~{N}-[[4-[[(2~{S})-4-cyclohexyl-1-[[(3~{S})-1-methylsulfonylpiperidin-3-yl]amino]-1-oxidanylidene-butan-2-yl]carbamoyl]phenyl]methyl]imidazo[1,2-a]pyridine-3-carboxamide 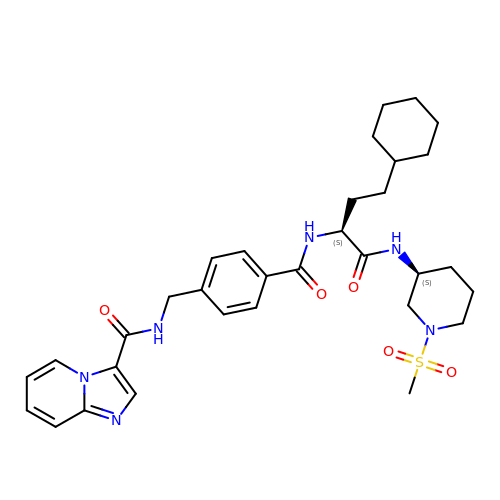| C32 H42 N6 O5 S | WGMNFJAFXXXRLZ-SVBPBHIXSA-N>SNASQSFMRTLGFLYGGRGMRSFLLNRKKKTAEGFRKIQGRDLIRIVFFEGVLYLNGLERKPKKLPRRFFNMVPLFSQLLRQHRRCPYSRLLQKTCPLVGIKDAGQAELSSFLPQHCGSHRVYLFVRECLLAVIPQ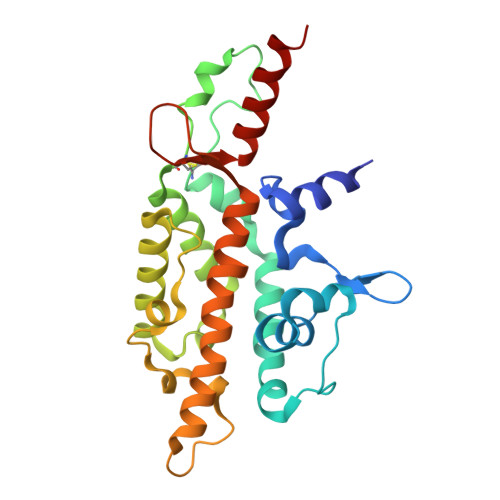ELWGSEHNRLLYFARVRFFLRSGKFERLSVAELMWKIKVNNCDWLKISKTGRVPPSELSYRTQILGQFLAWLLDGFVVGLVRACFYATESMGQKNAIRFYRQEVWAKLQDLAFRSHIS[4x]>RKPKTGILMLNMGGPETLGDVHDFLLRLFLDRDLMTLPIQNKLAPFIAKRRTPKIQEQYRRIGGGSPIKIWTSKQGEGMVKLLDELSPNTAPHKYYIGFRYVHPLTEEAIEEMERDGLERAIAFTQYPQYSCSTTGSSLNAIYRYYNQVGRKPTMKWSTIDRWPTHHLLIQCFADHILKELDHFPLEKRSEVVILFSAHSLPMSVVNRGDPYPQEVSATVQKVMERLEYCNP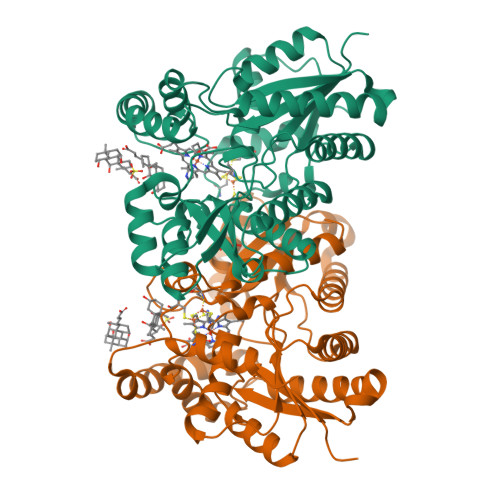YRLVWQSKVGPMPWLGPQTDESIKGLCERGRKNILLVPIAFTSDHIETLYELDIEYSQVLAKECGVENIRRAESLNGNPLFSKALADLVHSHIQSNELCSKQLTLSCPLCVNPVCRETKSFFTSQQL[2x]> MLPRETDEEPEEPGRR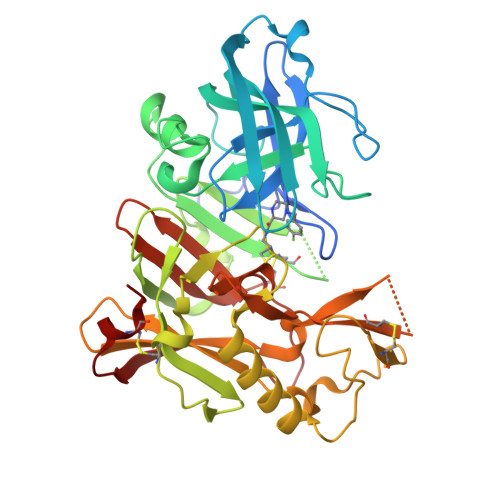GSFVEMVDNLRGKSGQGYYVEMTVGSPPQTLNILVDTGSSNFAVGAAPHPFLHRYYQRQLSSTYRDLRKGVYVPYTQGAWAGELGTDLVSIPHGPNVTVRANIAAITESDKFFINGSNWEGILGLAYAEIARPDDSLEPFFDSLVKQTHVPNLFSLQLCGAGFPLNQSEVLASVGGSMIIGGIDHSLYTGSLWYTPIRREWYYEVIIVRVEINGQDLKMDCKEYNYDKSIVDSGCTNLRLPKKVFEAAVKSIKAASSTEKFPDGFWLGEQLVCWQAGTTPWNIFPVISLYLMGEVTNQSFRITILPQQYLRPVEDVATSQDDCYKFAISQSSTGTVMGAVIMEGFYVVFDRARKRIGFAVSACHVHDEFRTAAVEGPFVTLDMEDCGYN N-[(benzyloxy)carbonyl]-O-tert-butyl-L-seryl-N-{(2R)-5-ethoxy-5-oxo-1-[(3S)-2-oxopyrrolidin-3-yl]pentan-2-yl}-L-phenylalaninamide 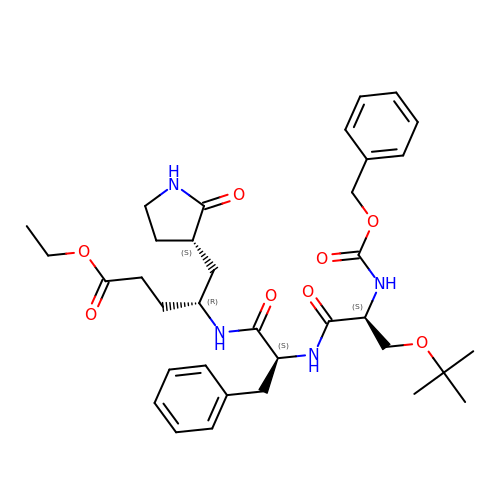| C35 H48 N4 O8 | JRBUWNJDFCUWEM-CRNKYVSFSA-N>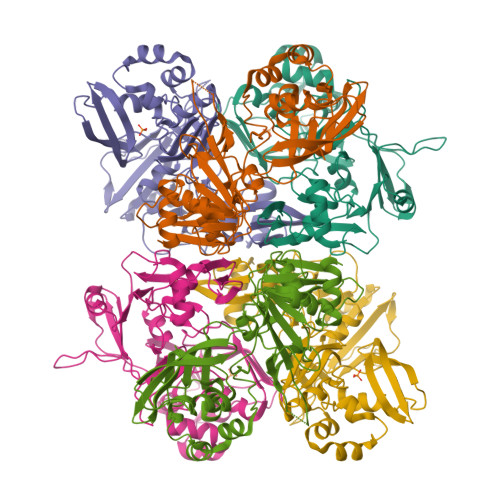[6x]SGLENIAFNVVNKGSFVGADGELPVAASGDKVFVRDGNTDNLVFVNKTSLPTAIAFELFAKRKVGLTPPLSILKNLGVVATYKFVLWDYEAERPLTSFTKSVCGYTDFAEDVCTCYDNSIQGSYERFTLSTNAVLFSATAVKTGGKSLPAIKLNFGMLNGNAIATVKSEDGNIKNINWFVYVRKDGKPVDHYDGFYTQGRNLQDFLPRSTMEEDFLNMDIGVFIQKYGLEDFNFEHVVYGDVSKTTLGGLHLLISQVRLSKMGILKAEEFVAASDITLKCCTVTYLNDPSSKTVCTYMDLLLDDFVSVLKSLDLTVVSKVHEVIIDNKPWRWMLWCKDNAVATFYPQLQ> GPLGSPEFNRPVKRMIALYDYDPQELSPNVDAEQVELCFKTGEIILVYG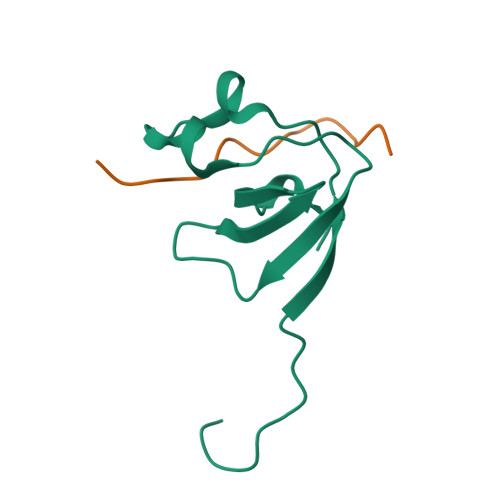DMDEDGFYMGELDGVRGLVPSNFLAD;> XIGRRLPPTPSKPSTLX> SNAEPSSKRRKHQGVIKRNWEYICSHDKEKTKILGDKNVDPKCEDSENKFDFSVMSYNILSQDLLEDNSHLYRHCRRPVLHWSFRFPNILKEIKHFDADVL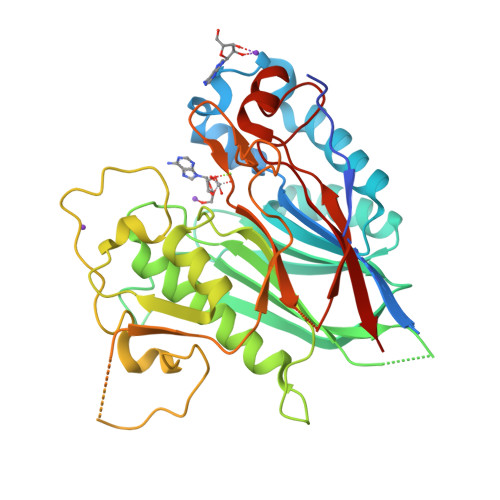CLQEVQEDHYGAEIRPSLESLGYHCEYKMRTGRKPDGCAICFKHSKFSLLSVNPVEFFRPDISLLDRDNVGLVLLLQPKIPYAACPAICVANTHLLYNPRRGDIKLTQLAMLLAEISSVAHQKDGSFCPIVMCGDFNSVPGSPLYSFIKEGKLNYEGLPIGKVSGQEQSSRGQRILSIPIWPPNLGISQNCVYEVQQVPKVEKTDSDLTQTQLKQTEVLVTAEKLSSNLQHHFSLSSVYSHYFPDTGIPEVTTCHSRSAITVDYIFYSAEKEDVAGHPGAEVALVGGLKLLARLSLLTEQDLWTVNGLPNENNSSDHLPLLAKFRLEL> SMSSKGSVVLAYSGGLDTSCILVWLKEQGYDVIAYLANIGQKEDFEEARKKALKLGAKKVFIEDVSREFVEEFIWPAIQSSALYEDRYLLGTSLARPCIARKQVEIAQREGAKYVSHGATGKGNDQVRFELSCYSLAPQIKVIAPWRMPEFYNRFKGRNDLMEYAKQHGIPIPVTPKNPWSMDENLMHISYEAGILENPKNQAPPGLYTKTQDPAKAPNTPDILEIEFKKGVPVKVTNVKDGTTHQTSLELFMYLNEVAGKHGV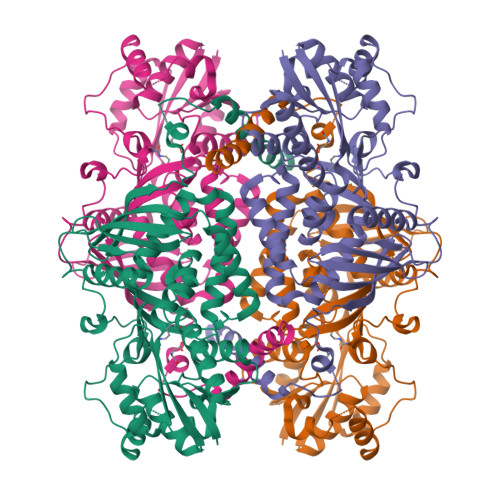GRIDIVENRFIGMKSRGIYETPAGTILYHAHLDIEAFTMDREVRKIKQGLGLKFAELVYTGFWHSPECEFVRHCIAKSQERVEGKVQVSVLKGQVYILGRESPLSLYNEELVSMNVQGDYEPTDATGFININSLRLKEYHRLQSKVTAK>DSVYVQNPQIPILVDRTDNVLFRIRIPDATKGDVLNRLTIRFGNEDKLSEVKAVRLFYAGTEAATKGRSRFAPVTYVSSHNIRNTRSANPSYSIRQDEVTTVANTLTLKTRQPMVKGINYFWVSVEMDRNTSLLSKLTSTVTEVV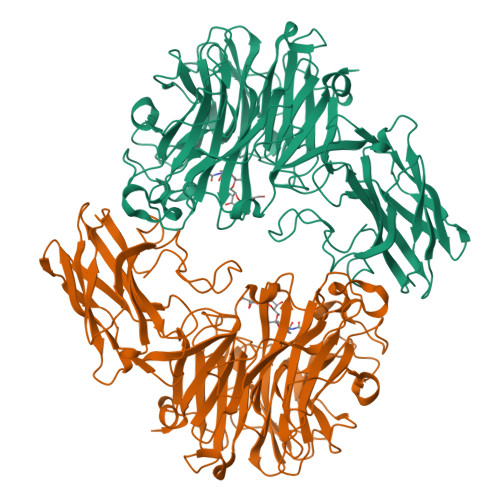INDKPAVIAGEQAAVRRMGIGVRHAGDDGSASFRIPGLVTTNKGTLLGVYDVRYNNSVALQEHIDVGLSRSTDKGQTWEPMRIAMSFGETDGLPSGQNGVGDPSILVDERTNTVWVVAAWTHGMGNARAWTNSMPGMTPDETAQLMMVKSTDDGRTWSESTNITSQVKDPSWCFLLQGPGRGITMRDGTLVFPIQFIDSLRVPHAGIMYSKDRGETWHIHQPARTNTTEAQVAEVEPGVLMLNMRDNRGGSRAVSITRDLGKSWTEHSSNRSALPESICMASLISVKAKDNIIGKDLLLFSNPNTTEGRHHITIKASLDGGVTWLPAHQVLLDEEDGWGYSCLSMIDRETVGIFYESSVAHMTFQAVKIKDLIR[2x]>[2x]UUGCGU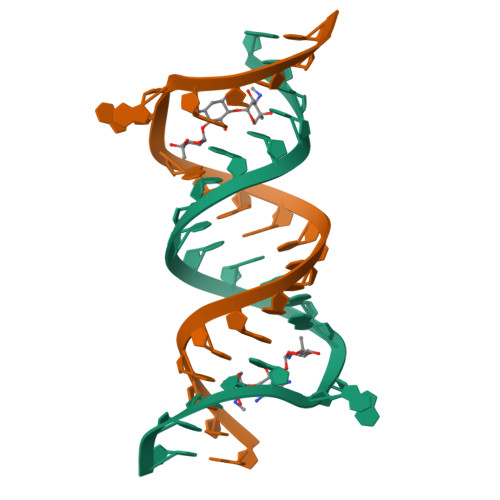CGUUCCGGAAAAGUCGC The papillomaviruses (PV) are small dsDNA tumour viruses of significant medical importance and the prototype of the group is bovine PV (BPV-1). The N-terminal half of BPV-1 E1 consists of a regulatory domain (residues ∼1–158) and a sequence specific origin of replication (ori) DNA binding domain (ori binding domain; OBD, residues ∼159–300), implicated in replication initiation. The C-terminal half (residues ∼301–605, the E1 helicase domain—E1HD) has helicase activity and can be sub-divided into the oligomerization domain (OD, residues ∼308–378) and the AAA+ adenosine triphosphatase (ATPase) domain that includes a flexible C-terminal acidic tail (AT, residues 579–605) required for helicase processivity. Crystal structures of the E1HD show hexamers with two tiers formed by the OD and the AAA+ domain.

To advance understanding of the mechanism of dsDNA strand separation we have used electron microscopy (EM) and single particle analysis to obtain structures of the full length BPV helicase E1 and two complexes of E1 bound to a RFJ end-labelled with protein tags. First, a structure of the purified E1FL–T30 complex examined by negative stain EM was determined with C6 rotational symmetry imposed during the initial structure determination. The E1FL hexamer structure, determined at a resolution of 18 Å, has a maximum diameter of 130 Å and a height of 100 Å and can accommodate ∼410 kDa of protein mass, in agreement with the predicted 409 kDa. The shape of the complex resembles a triple-tiered ring, with the middle ring having the larger diameter and the upper ring the smallest (left). There is a central tunnel (‘a’) that varies in diameter along its length: at the bottom of the structure (C-terminus) the tunnel is ∼20 Å in diameter; travelling upwards the tunnel ‘a’ forms a chamber within the HD area, which expands to 27 Å below sub-domain 3 (middle) and then it narrows to 23 Å in diameter at the entrance to the central tunnel formed by the upper ring. Third, available atomic coordinates of E1 domains were docked into the EM maps. The fitting resulted in a CCC = 0.72, which was reduced to ∼0.2 for the upper tier of the complex indicating a better consistency between E1HD crystal structures and the lower tiers of the E1FL structure. Notably, the data indicate that dsDNA enters the E1 complex through a tight side tunnel and not along the central axis of the hexamer as commonly assumed for E1 and other hexameric helicases, while the 5′ ‘passive’ strand exits the complex via a channel opposite the dsDNA entry tunnel. DNA unwinding is therefore taking place at the entrance to the helicase domain, inside and not outside the hexamer. Our observations therefore suggest a revision of the steric exclusion model proposed for E1 (20) where, alternatively, DNA strands are wedged apart within the hexameric assembly and not outside.

>TLNESLQTEKFDFGTMVQWAYDHKYAEESKIAYEYALAAGSDSNARAFLATNSQAKHVKDCATMVRHYLRAETQALSMPAYIKARCKLATGEGSWKSILTFFNYQNIELITFINALKLWLKGIPKKNCLAFIGPPNTGKSMLCNSLIHFLGGSVLSFANHKSHFWLASLADTRAALVDDATHACWRYFDTYLRNALDGYPVSIDRKHKAAVQIKAPPLLVTSNIDVQAEDRYLYLHSRVQTFRFEQPCTDESGEQPFNITDADWKSFFVRLWGRLDLIDEEEDSEEDGDSMRTFTCSARNTNAVD[6x]> 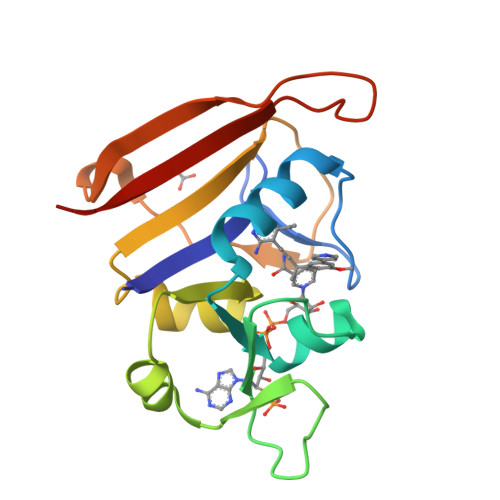MTLSILVAHDLQRVIGFENQLPWHLPNDLKHVKKLSTGHTLVMGRKTFESIGKPLPNRRNVVLTSDTSFNVEGVDVIHSIEDIYQLPGHVFIFGGQTLFEEMIDKVDDMYITVIEGKFRGDTFFPPYTFEDWEVASSVEGKLDEKNTIPHTFLHLIRKLE> QDADKLPHTKVTLVAPPQVHPHEQASKTGPKVVEFTMTIEEKKMVIDDKGTTLQAMTFNGSMPGPTLVVHEGDYVQLTLVNPATNAMPHNVDFHGATGALGGAKLTNVNPGEQATLRFKADRSGTFVYHCAPEGMVPWHVVSGLSGTLMVLPRDGLKDPEGKPLHYDRAYTIGEFDLYIPKGPDGKYKDYATLAESYGDTVQVMRTLTPSHIVFNGKVGALTGANALTAKVGETVLLIHSQANRDTR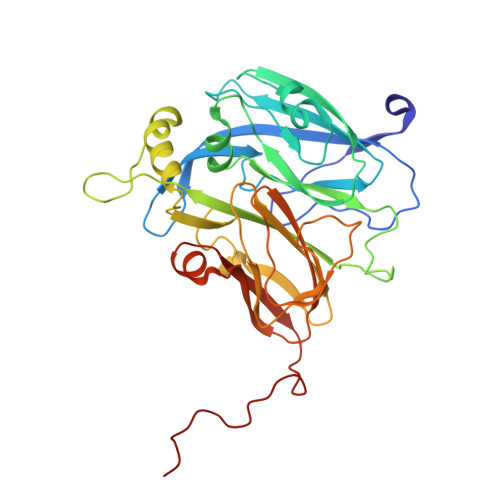PHLIGGHGDWVWETGKFANPPQRDLETWFIRGGSAGAALYTFKQPGVYAYLNHNLIEAFELGAAGHIKVEGKWNDDLMKQIKAPAPIPR>[2x]MGHESDELNPEPLTDLNQLPVQV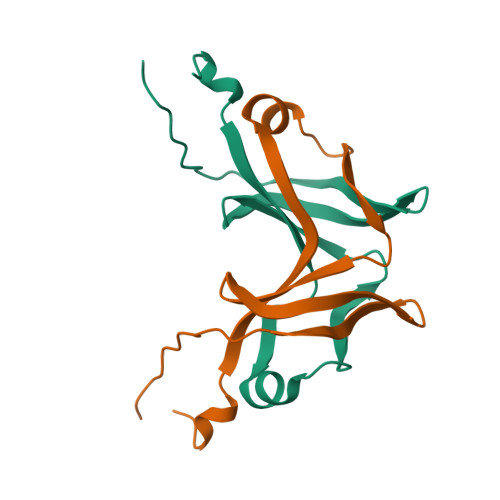SFEVGRQILDWHTLTSLEPGSLIDLTTPVDGEVRLLANGRLLGHGRLVEIQGRLGVRIERLTEVTISLEVLFQ> MGSSHHHHHHSSGENLYFQGHMIRIGVLISGSGTNLQAILDGCREGRIPGRVAVVISDRADAYGLERARRAGVDALHMDPAAYPSRTAFDAALAERLQAYGVDLVCLAGYMR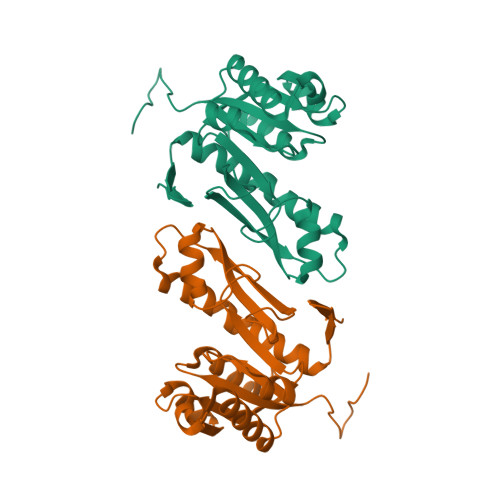LVRGPMLTAFPNRILNIHPSLLPAFPGLEAQRQALEHGVKVAGCTVHFVTAGVDEGPIILQAAVPVLEGDTVEDLRRRILAEEHRIYPEAIRLFAEGRLVIEGRRVRILDRAEAPRG>MDHHHHHHDTGQSQTQRMYNYLKAKYTATSGTQLAWGAYLDPVDGNPSSVYAEFDERAHNVDPSTEPIKSTHTFKDGSVAEIEMNGQLVDGLTGPENYNITIKSKSKLAGSNDYYEHIVTFNFDTKGIRSEEGHLRSAQK[4x]

Type 4 pili (T4P)—important in bacterial pathogens—are filaments composed of one well-characterized major pilin, and several minor pilins whose roles are often poorly understood. Streptococcus sanguinis T4P are composed of five pilins, which makes it a good model to determine the role of each pilin subunit in detail. PilE1/PilE2 are the major pilins forming the backbone of the filament, while the three minor pilins (PilA, PilB, and PilC) form a tip-located complex promoting adhesion to various host receptors. Here, we characterize PilA and PilC, showing how they interact and how they function.

Although it has a typical pilin size—17 kDa for the processed protein—PilA is an unusual pilin. To better understand the role of PilA, we solved its 3D structure by X-ray crystallography. After optimizing the best diffracting crystals and using protein produced in the presence of seleno-methionine (SeMet) for phase determination, we solved a 1.77-Å resolution structure. As can be seen in Fig. 2A, PilA—which looks like an “ice axe”—exhibits a typical pilin architecture, with an N-terminal α1-helix packed against a β-sheet composed of five antiparallel β-strands. A closer inspection of the crystal packing showed that PilA forms head-to-toe dimers, stabilized by a series of hydrogen bonds between residues in α1-helix and the last two β-strands of the β-sheet (β4 and β5). Strikingly, while PilA exhibits no sequence homology to other pilins, our structure reveals extensive structural similarity to the I subunit of HIJK tip-located complex of conserved minor pilins in a variety of T4F. Critically, since I interacts with J and K, this suggested to us that PilA might be interacting with another minor pilin (PilB and/or PilC) to form a complex capping S. sanguinis T4P. Using isothermal titration calorimetry (ITC), we showed that PilA has high affinity for PilC, with a dissociation constant (KD) of 23.8 ± 7.9 nM. The PilAC interaction interface involves the α1 and α2 helices and the first 2 β-strands (β1 and β2) of PilA. PilA thus acts as an intrapilus chaperone, protecting PilC from proteolysis by perhaps participating in its folding.>[2x]GAMDDSSLQKVELQTDVYMVCLQHALSTENFEVMGLLIGNFACGIAKISAVIILRRLDKKKDRVEISSEQLLKAAAEAERLTVELNRPMRVLGWYHSHPHITVCPSHVDVRTQATYQTMDHSFVGLIFSVFSEGKESKEHEIFLNCFQSDNGEATEIPLEIVHTPDISDRCLRTMTDLSKILVQEEEDMAEACKDHPDVLASIHNNAVRTRALIHITDIITKPLVQTFEKRIALNKLRATHLQRQLQELQKMCNG;>[2x]MADSDLLVTISGAALSLLFFENVRSVGNQMGFLLGEALEFIVKTYTDSDNQVETVKIHINVEAIVTCPLADLLHDSTNHINKEKLKDFVRDKSKQVIGWFCFRRNTTNLTLTLKDKLLHKQFASHFSGVNGCKEDFFLTCLLNASTSETSGTHKFRHVFLRHNKRGMFEPISLKINNLGDDASRHDGSDYKPTPVRKSTRTPDSFTKLIESLNLDVARIDGLDSAMLIQKAAEHHLMSLIPKVCESDLEVAELEKQVHELKIKIATQQLAKRLKINGENCDRISKASKD

BRCC36 is the catalytic subunit responsible for the majority of K63-Ub specific DUB activity in the cytoplasm and in the nucleus as part of two distinct macromolecular assemblies characterized by the presence of either of the MPN− pseudo DUB proteins KIAA0157 or Abraxas. The Abraxas complex (ARISC) functions in DNA repair and breast cancer suppression, while the BRCC36 isopeptidase complex (BRISC) promotes interferon dependent responses by deubiquitinating and stabilizing the type I interferon receptor, IFNAR1. BRCC36 consists of a functional metalloprotease JAMM/MPN+ domain followed by a predicted coiled coil region implicated in protein-protein interactions. KIAA0157 and Abraxas are required for the catalytic function of BRCC36 in both complexes, and enable association of two additional shared subunits (BRCC45 and MERIT40) to each holoenzyme.

Optimization of the CfKIAA0157 construct boundaries by deletion of poorly conserved C-terminal residues 290 to 471 (CfKIAA0157ΔC) yielded crystals in complex with full length CfBRCC36 (residues 1-253) that diffracted to 2.55 Å resolution. We solved the CfBRCC36–KIAA0157ΔC crystal structure using the seleno-methionine-SAD method (See Methods for seleno-methionine protein production and crystallographic details). Following manual rebuilding and refinement, two highly interdigitated CfBRCC36–KIAA0157ΔC heterodimers were apparent in the asymmetric unit, arranged in the suspected super dimer configuration. The final model displayed good crystallographic and geometric statistics (Rwork/Rfree = 0.189/0.240; see Table 1 for data collection and refinement statistics). The structure of each protomer of CfBRCC36 and CfKIAA0157 consisted of a canonical MPN domain (residues 1–165 in BRCC36 comprising an eight strand β-sheet flanked by three α-helices and residues 1–180 in KIAA0157 comprising a seven strand β-sheet flanked by three α-helices), followed by two non-canonical helices α4 and α5 within the predicted coiled coil regions. CfBRCC36 and CfKIAA0157ΔC protomers heterodimerized through a large buried surface area (SA) of 8112 Å2. The MPN domains of each associated in a pseudo two-fold manner centered on helices α1, resulting in a unified β-sheet and “fused” MPN+–MPN− superstructure (buried SA = 2902 Å2). Non-canonical helices α4 and α5 of CfBRCC36 interacted with helices α4 and α5 of CfKIAA0157 in the form of a coiled coil helical bundle (CCHB). Ab initio modeling and comparison of the calculated scattering curves for the heterodimer and the four possible super dimers with the experimental data using CRYSOL was most consistent with the two-fold symmetric super dimer configuration centered on CfBRCC36 helix α5 that buried 3093 Å2 of surface area. Contacts were predominantly hydrophobic in nature involving reciprocal patches composed by Leu198, Ile201, Ala205 and Ile212 side chains on opposing CfBRCC36 protomers.> GSARENEMDENLEQVS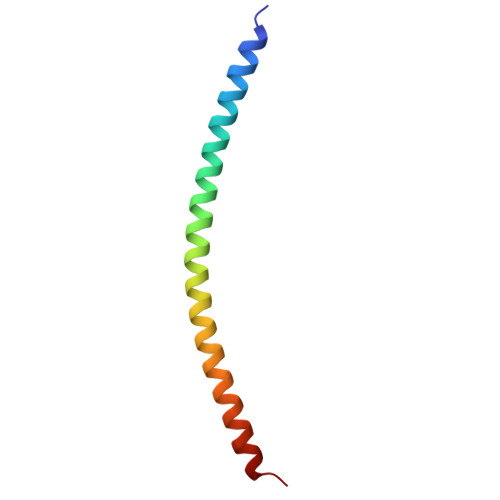GIIGNLRHMALDMGNEIDTQNRQIDRIMEKADSNKTRIDEANQRATKMLG>MIKELHVKTVKRGENVTMECSMSKVKDKNKLAWYRQSFGKVPQYFVRYYSSNSGYKFAEGFKDSRFSMTVN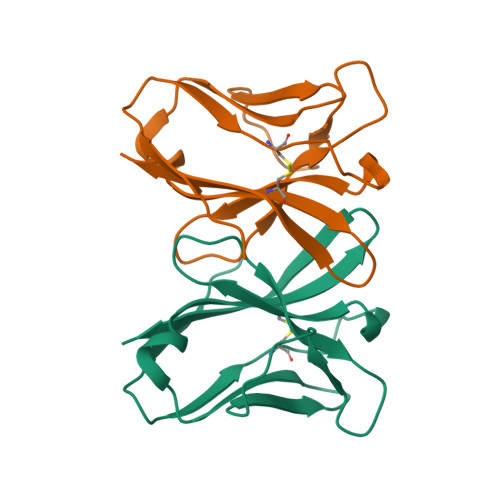DQKFDLNIIGTREDDGGEYFCGEVEGNTIKFTSGTRLQF[2x]The evolutionary arms race between prokaryotes and phages gave rise to phage anti-CRISPR (Acr) proteins that act as a counter defence against CRISPR-Cas systems by inhibiting the effector complex. Here, we used a combination of bulk biochemical experiments, X-ray crystallography and single-molecule techniques to explore the inhibitory activity of AcrIF6 and AcrIF9 proteins against the type I-F CRISPR-Cas system from Aggregatibacter actinomycetemcomitans (Aa). The biochemical analysis revealed that both AcrIF6 and AcrIF9 interact with the Aa-Cascade complex and interfere with the DNA target recognition; however, AcrIF9 binding to Aa-Cascade also stimulated non-specific DNA binding. The cryo-EM structures of Pa- and Pp-AcrIF9 bound to the Pa-Cascade complex indicate that two AcrIF9 molecules bind to the thumbs of Cas7f.4 and Cas7f.6 subunits and the two AcrIF9 binding sites are similar.

We solved the crystal structure of Aa1-AcrIF9 protein at 2.3 Å resolution. Aa1-AcrIF9 is composed of a five stranded, antiparallel β sheet cradling an α helix. We superimposed the structures and identified the Aa1-AcrIF9 surfaces potentially involved in the interactions with Cas7f subunits and DNA. The positively charged surface can be observed within the structure of the Aa1-AcrIF9 protein. Mutational analysis of this surface proved that it is the binding site for the non-specific DNA. The M1, M2, and M3 mutations disrupted the AcrIF9-mediated binding to non-specific DNA as the smeared DNA bands disappeared in EMSAs with target and non-target DNA. The M4 and M5 mutations of Aa1-AcrIF9 permitted the Cascade binding to the target sequence leading to unhindered R-loop formation and the Cas2/3-mediated cleavage. The deletion of the L3-4 loop (M6) or its replacement with the Pa-AcrIF9 loop (M7) completely blocked the Aa1-AcrIF9 interaction with the Cascade. However, the stability of these mutants was substantially lower than WT or other Aa1-AcrIF9 mutants. This indicates that the L3-4 loop plays an important structural role within Aa1-AcrIF9 and most likely participates in interaction with the Cascade complex.

> MGSSHHHHHHSQDPMTNVVYYFTETNNINAYATAEALKAQTLADAKREASRRQCFQGTTLKIGTIYSLNSDGLLVDEITSKEDGKKWVDRY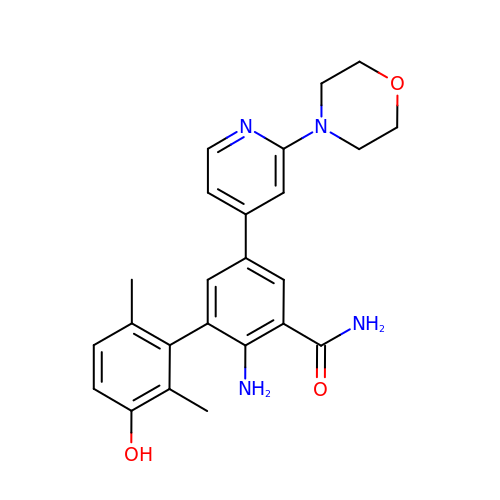2-azanyl-3-(2,6-dimethyl-3-oxidanyl-phenyl)-5-(2-morpholin-4-ylpyridin-4-yl)benzamide | C24 H26 N4 O3 | YNPXBUGWZQVVNF-UHFFFAOYSA-N> MSPILGYWKIKGLVQPTRLLLEYLEEKYEEHLYERDEGDKWRNKKFELGLEFPNLPYYIDGDVKLTQSMAIIRYIADKHNMLGGCPKERAEISMLEGAVLDIRYGVSRIAYSKDFETLKVDFLSKLPEMLKMFED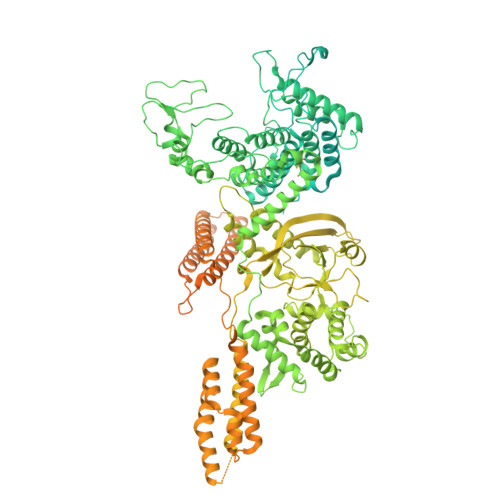RLCHKTYLNGDHVTHPDFMLYDALDVVLYMDPMCLDAFPKLVCFKKRIEAIPQIDKYLKSSKYIAWPLQGWQATFGGGDHPPKSDLEVLFQGPLGSMPKYVEGVELTQEGMHAIFARMGHGDITSGSIYNGVPTIDTEALNRQGFMPVLTGVGPRRDSGHWIMLIKGPGNQYFLFDPLGKTSGEGYKNTLLAQLPIASTLSVIPNEPGLNKGLCGYWVASVGLKARSELSKDNPPNLETLGQITTDAMKDELTDNGYLKITGWLKAVADKFPEGDPQPDAKALRQTTEKDLHIEIPSPVSPIKDTAPKEVSTKPTAPQVAPKHSLDSKLLENDDDVLDTIKYVHKEYLGKPYPGPLKNPKAPEEGRLPPNEGPDRGPHGLAHTVRTMACAEVMIEEARKAQLRGETLGKAKNGQTLADVTPEELKKILIAQAFFVVGRDDERSGYDDVHKRNFYAEYHEKSEQAFRKYVEDNKLIGKIFKDQKEVDFYAAIILDKNHEWDATPAHILINQGHMVDLMRTKAPAEVALERTYNTLKGTVGSKGAEVVLKAHRDFFFATGAVVPLVNPEAIDDPSRGGPYENPYSGEKFVIVDDKVPASKKDLPKAVNRDYKLKDNERFLTIKEYYAFPDVQQTYPGYKTRLEASSYYFPTPFAGECEQNPAKCLGAIQKARSKLQTDAIKNGFQSSSEKERRQPNMDEIAAARIIQQIMANPDCIHDDHVLINGQKLEEKFFRDLLAKCDMAVVGSLLNDTDIKNIDTLMRHEKNTEFHSTDPKAVPVKIGDAWENRIRTKGGDVTQMKHDLIFLMQNDAWYFSRVNAIAQNRDKGSNFKEVLFTTLMTPLTNKSLIDTSHVPAPKKLYRGLNLPQEFTNKLINQSNAIIANTENTLFTDLSAEAFKQIKLNDFSQMSGKTCASTTKNMKLLTDIWGSNVIFEMLDPDGLLHPKQVGTHMAGSEDEFSVYLPEDVALVPTKVTLEGKTDTGEDRYIFTLVAVKSPDFIPRHESGYAVEPFMKMQKEKVTQALDAIEKDKDSYNIDEQLKSLRTEMVRQAKLPLREGVFDRLSHRLSLETSDNKISPERRDFLNQHVIPVLQECHIALRANDMDMMQKALAKFPTDKQWSAFKSGEAVRAKAQMDVLKQQIEKKIMLQTQIIPALTECGEALDKQNVTEALQALNKLPAEKEIGKVKTIGQELRGQIVGVKQELTGNLEPLQRATTTPIVQDAEKIKVRYETLLTDVTKRVTDFEKIKPANLDGYNKAIADLNNIQQELNLLRNEKIRMHTDKDKAVDFSDIEALDKRLQDVQSKLPTQLLEQTSKDVAKLAKMPEKITFNDIKSMTSKMNNYLETLELIRNDRIKKHAGSTDPLDMSDLDGLKGQLQTYNQSMADILLRAAKSSLDKIKDPATFEKESPYIKQCFDHLAELEKTLDDSDKGRKQKEDFTAYKSALMDKQEKAYPEMLQLQYKSEALIMQLRDICKIHHDNLAEARRVRLQQLDSQGGGLLGGLWAVTNTIGLTTDNVNIEKMQIRMKEQTLRAFKTELTNDKLNTDQVIAFLAKGSPSELQEALGISKENAEQLHGLLKQLEIKTASTDKLQEIEKLIDEVSTKIGKEPVKQDHTITIDEEESDDIRYGF2-[2-[[3-[3-[(1~{S})-1-azanyl-2-oxidanyl-ethyl]phenyl]phenyl]methoxy]phenyl]ethanoic acid | C23 H23 N 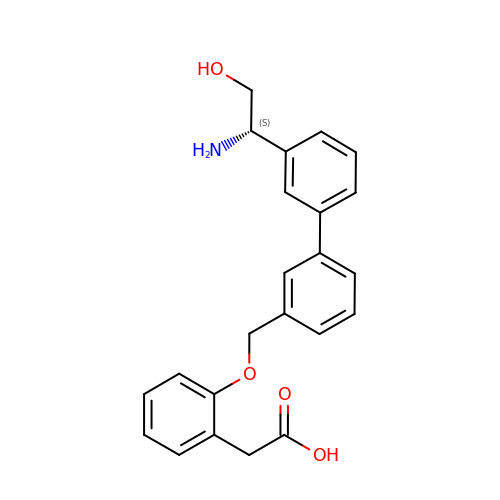O4 | XHLXBWRISOPXQB-OAQYLSRUSA-N>GHMETGDQRFGDLVFRQLAPNVWQHTSFEEVNGWGVVPSNGLIVRDGGRVLVVDTAWTDDQTAQILNWIKQEINLPVALAVVTHAHQDKMGGMDALHAAGIATYANALSNQLAPQEGMVAAQHSLTFAANGWVEPATAPNFGPLKVFYPGPGHTSDNITVGIDGTDIAFGGCLIKDSKAKSLGNLGDADTEHYAASARAFGAAFPKASMIVMSHS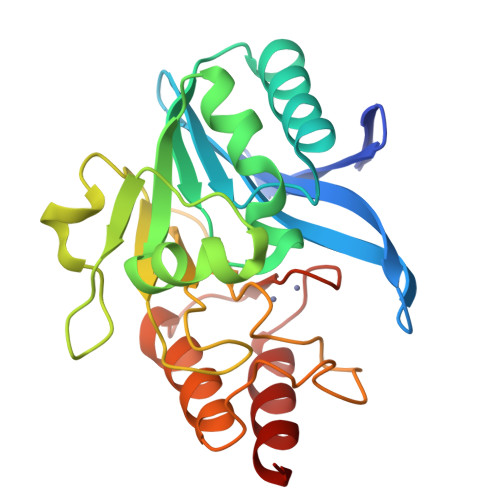APDSRAAITHTARMADKLR[2x]>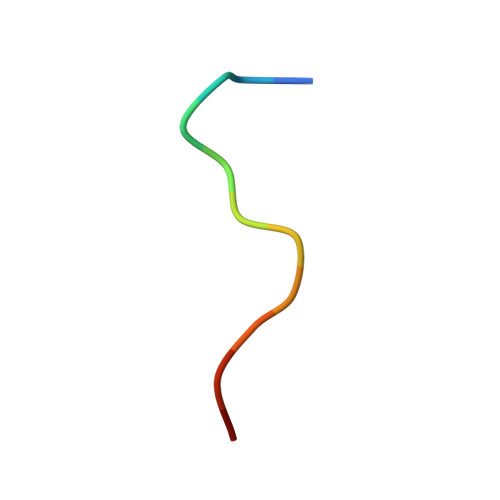 QRPTQPVYQIQN2-PHENYLMALONIC ACID | C9 H8 O4 | 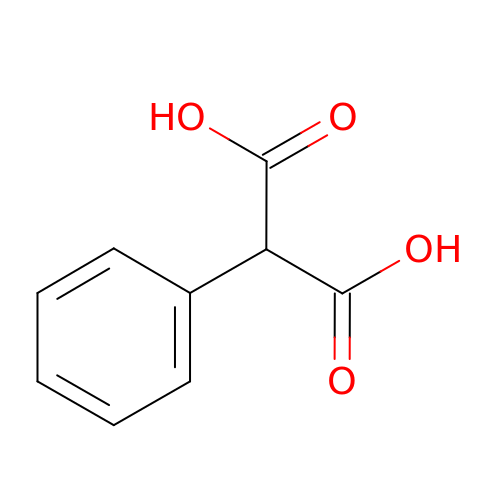WWYDYZMNFQIYPT-UHFFFAOYSA-N>MKAKIFSGVIPALMTPGREDRTPDFDALVRKGKALIADGMSAVVYCGSMGDWPLLTDAQRMEGVERLVKAGVPVIVGTGAVNTALAAAHAAHAQKVGAQGLMVIPRVLS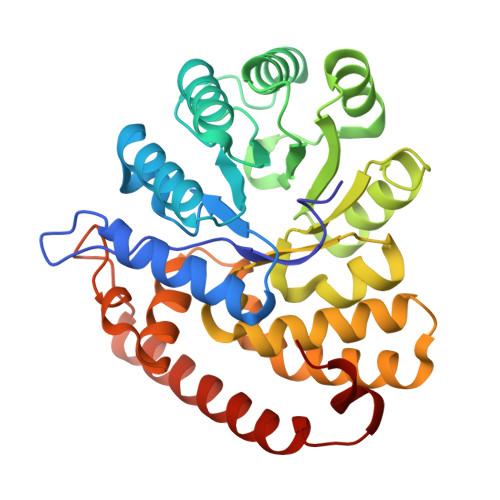RGPSIVAQKAHFKAILAAAPDLPSVIYNSPYYGFATRADLFFALRAEHPNLVGFKEFGGNADMRYAAEHITSRDDGVSLMIGVDTAVFHGFVNCGATGAITGIGNVLPKEVIHLCNLSRAAAAGDVDARQRAQELEQALAVLSSFDEGPDLVLYFKHMMVLKGDKEYTLHFNETDALTESQRGYVEAQFKLFNTWYAEWSKLPGAVEKYKA[2x]>GPEEERAFLVAREELASALRRDSGQAFSLEQLRPLLASSLPLAARYLQLDAARLVRCNAHGEPRNYLNTLSTALNILEKYGRNLLSPQRPRYWRGVKFNNPVFRSTVDAVQGGRDVLRLYGYTEEQPDGLSFPEGQEEPDEHQVATVTLEVLLLRTELSLLLQNTHPRQQALEQLLE[2x];>[2x]AEHEEDMYRAADEIEKEKE

The linear ubiquitin (Ub) chain assembly complex (LUBAC) generates Met1-linked “linear” Ub chains that regulate the activation of the nuclear factor κB (NFκB) transcription factor and other processes. (2006) identified the linear Ub chain assembly complex (LUBAC), which consists of the chain-assembling E3 ligase HOIP as well as HOIL-1 and SHARPIN (Walczak et al., 2012). HOIP also comprises several NPL4 zinc finger (NZF) Ub binding domains (UBDs) that target it to ubiquitinated proteins (Haas et al., 2009), a Ub-associated (UBA) domain that mediates interactions with HOIL-1 (Yagi et al., 2012), and N-terminal PUB (peptide:N-glycanase/UBA- or UBX-containing proteins) and B box domains of unknown functions. Here, we show that OTULIN interacts directly with the N-terminal PUB domain of HOIP via a conserved PUB-interacting motif (PIM) in OTULIN.

We determined the structure of a slightly truncated HOIP PUB domain construct (aa 5–180) bound to the OTULIN PIM peptide (aa 49–67) to 2.0 Å resolution. The two molecules in the asymmetric unit were highly similar to the apo structures (rmsd ∼1.5 Å), which was consistent with NMR analysis. Both HOIP molecules showed similarly well-defined electron density for residues 53–65 of the PIM peptide. In analogy to the p97-PNGase interaction, only PIM residues 54–58 interact with HOIP. The PIM peptide forms a 90° kink, in which Met55 and Tyr56 form a bulge and mediate key hydrophobic interactions. As expected, the OTULIN PIM peptide binds to the conserved PIM pocket in the HOIP PUB domain. The key PIM residue Tyr56 is buried in a pocket formed by Tyr82 (αA), Tyr124, and Pro92 and formed a hydrogen bond with Asn85 from HOIP. The second hydrophobic PIM residue, Met55, is bound in a shallower groove between HOIP PUB domain residues Tyr82, Ile78 (αA), and Val104 (αB). More importantly, Asn102 in the PUB domain acts as the cornerstone around which the peptide is wrapped and interacts with the very same backbone of Asp54, Tyr56, and Arg57. Arg57 of the PIM peptide participates in a π-π stacking network with HOIP Tyr94, which is the only residue that undergoes a significant conformational change within the PIM pocket.>[2x]SMPTPEAPYASLTEIEHLVQSVSKSYRETCQLRLEDLLRQRSNIFSREEVTGYQRKSMWEM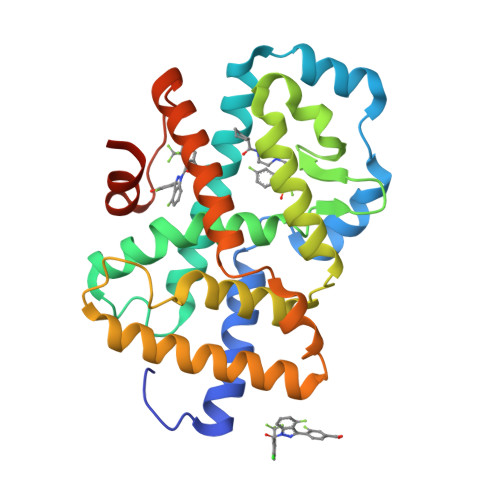WERCAHHLTEAIQYVVEFAKRLSGFMELSQNDQIVLLKAGAMEVVLVRMCRAYNADNRTVFFEGKYGGMELFRALGCSELISSIFDFSHSLSALHFSEDEIALYTALVLINAHRPGLQEKRKVEQLQYNLELAFHHHLCKTHRQSILAKLPPKGKLRSLCSQHVERLQIFQHLHPIVVQAAFPPLYKELFSTETESPVGLS> MGSKSKVDNQFYSVEVGDSTFTVLKRYQNLKPIGSGAQGIVCAAYDAVLDRNVAIKKLSRPFQNQTHAKRAYRELVLMKCVNHKNIISLLNVFTPQKTLEEFQDVYLVMELMDANLCQVIQMELDHERMSYLLYQMLCGIKHLHSAGIIHRDLKPSNIVVKSDCTLKILDFGLARTAGTSFMMTPYVVTRYYRAPEVILGMGYKENVDIWSVGCIMGEMVRHKILFPGRDYIDQWNKVIEQLGTPCPEFMKKLQPTVRNYVENRPKYAGLTFPKLFPDSLFPADSEHNKLKASQARDLLSKMLVIDPAKRISVD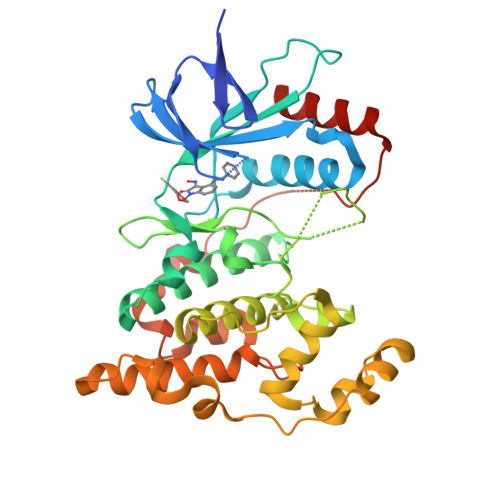DALQHPYINVWYDPAEVEAPPPQIYDKQLDEREHTIEEWKELIYKEVMNSE5-amino-3-(furan-2-yl)-1H-1,2,4-triazole-1-carboxamide 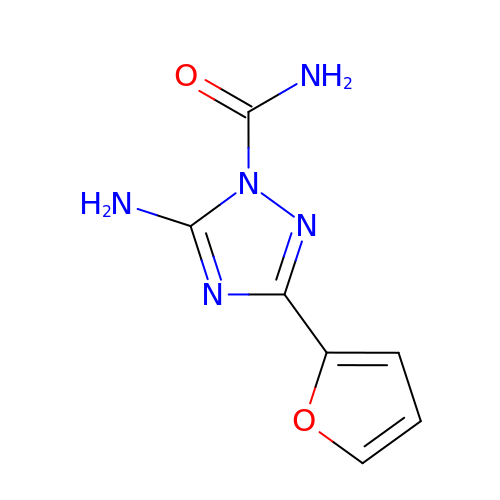| C7 H7 N5 O2 | NBDYCQJTOKDLCM-UHFFFAOYSA-N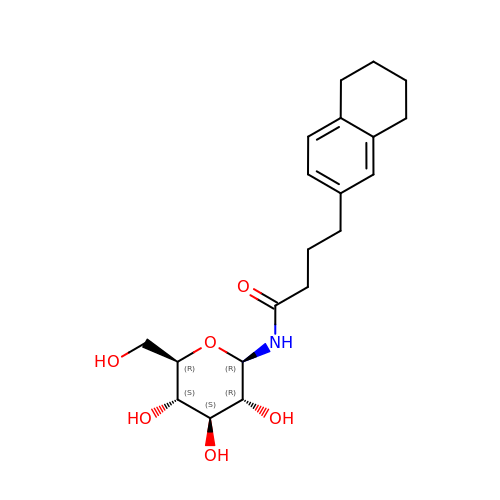N-[4-(5,6,7,8-tetrahydronaphthalen-2-yl)butanoyl]-beta-D-glucopyranosylamine | C20 H29 N O6 | XAFXSLABZKEYPA-XIKSMUEASA-N>SMFNNELMADVHFVVGPPGATRTVPAHKYVLAVGSSVFYAMFYGDLAEVKSEIHIPDVEPAAFLILLKYMYSDEIDLEADTVLATLYAAKKYIVPAL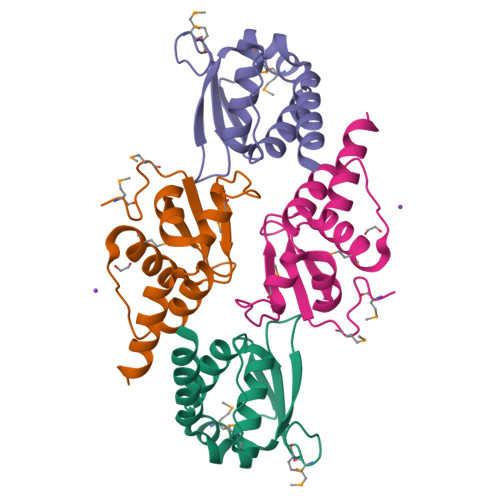AKACVNFLETSL[2x]>[2x]APPRKVLII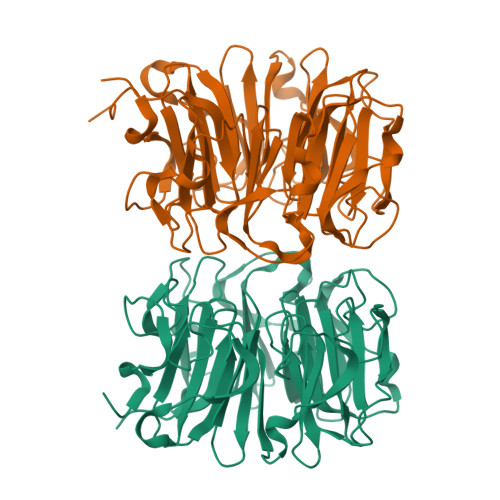SAGASHSVALLSGDIVCSWGRGEDGQLGHGDAEDRPSPTQLSALDGHQIVSVTCGADHTVAYSQSGMEVYSWGWGDFGRLGHGNSSDLFTPLPIKALHGIRIKQIACGDSHCLAVTMEGEVQSWGRNQNGQLGLGDTEDSLVPQKIQAFEGIRIKMVAAGAEHTAAVTEDGDLYGWGWGRYGNLGLGDRTDRLVPERVTSTGGEKMSMVACGWRHTISVSYSGALYTYGWSKYGQLGHGDLEDHLIPHKLEALSNSFISQISGGWRHTMALTSDGKLYGWGWNKFGQVGVGNNLDQCSPVQVRFPDDQKVVQVSCGWRHTLAVTERNNVFAWGRGTNGQLGIGESVDRNFPKIIEALSVDGASGQ(1R,2S,3S,4R)-5-METHYLENECYCLOHEXANE-1,2,3,4-TETRAOL 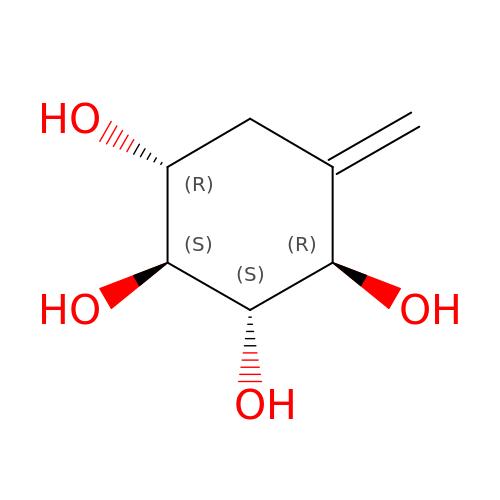| C7 H12 O4 | DRZDCPGIBPDBFY-JWXFUTCRSA-N>[12x]MSVIRIKTNAAVAAVLPANEDQADYPSTFFEGGNEIRLYVNRGE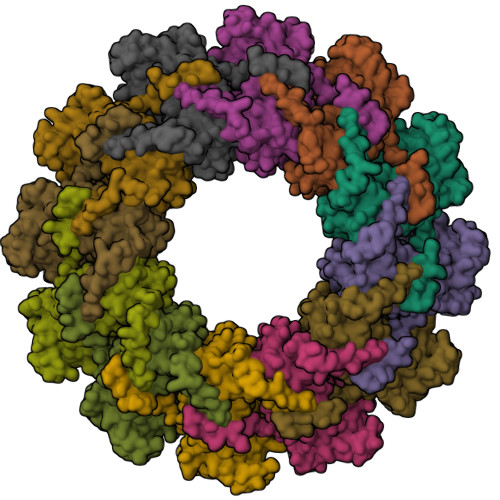KLDVLRQYVYMGLVEKNCRIQHVNAYLYAVLKGERELLEADWDSFGHKIGIQGDKIGPFNLVRVEDIPDGLPDGKLNAEVSAEDDAWLPLFLLGLYRVGRASETAYRTLLMESLIKQCKAIKSDWVSPVTATHKYFDVWGNDGNYLKIVACVDMFYNHFKKSIKATFRWGTIVSRFKDCAALATLGHVVKITGLTIEEVFTWVLQTEVADELVKMMKPGQEIDKSTSYMPYLIDMGISAKSPYSTIKNPSFHFWGQLVAALCRSKRALNARQPDEIDSMSISNASLLMAYALGSSPDIEQQFSTGNTYRKPPKEASYLVSEEPKNRSVVEWIAWYSDVDNKPTDDMLMMAKRVAGTISGPRDNSVGKWIKQTYG> GMGYTLAEFLAHAIALETEAAERYVELADMMEAHNNLDTATVFRDMARFSTLHGDEIKQRSRALELPKLMSWQYRWKTPPEVGDENDIHYLMTPYHALRYARDNEIRGMEYYKEAAANSADPEVKR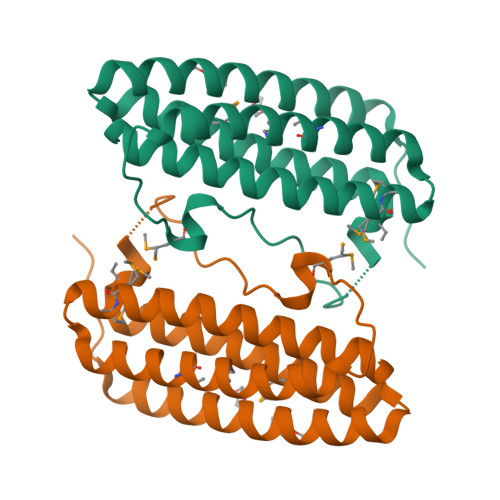LGADFAAEEAEHVVALDKWIEKTPRPSITWSEDADPAQCVD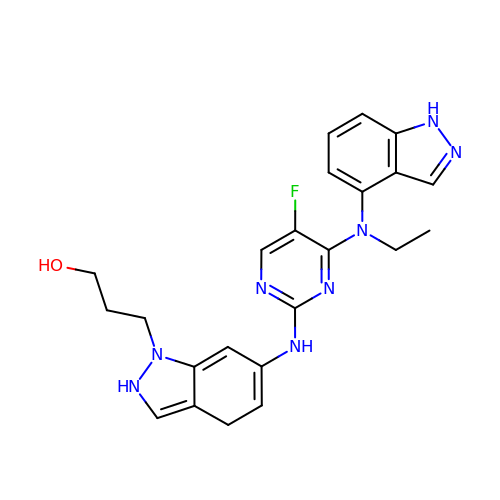3-[6-({4-[ethyl(1H-indazol-4-yl)amino]-5-fluoropyrimidin-2-yl}amino)-2,4-dihydro-1H-indazol-1-yl]propan-1-ol | C23 H25 F N8 O | WTARZSVAAGFJEN-UHFFFAOYSA-N>GGHMGAIVILVVGPPGSGKSQLIKAIEKLAREQGQPVVTTSVTSEDEAKKVLEELLKKDPNAIVVIEIKNPRIAERVAKRVLEEDPTAVLVVVVSSPEVARELRENLPNVIVVVLIRDPEKLKEAKKQGTQVLSGDGNPEEAAKQIAQLIKDQAGSWS[2x]

Here, we attempted to design an ATPase de novo, through the exploration of an optimal backbone blueprint to incorporate a conserved phosphate binding motif, the P‐loop, into designed structures. Many naturally occurring ATPases (Saraste et al., 1990; Walker et al., 1982) possess the P‐loop motif, with a sequence pattern of GX1X2X3X4GK[T/S] (X indicates any kind of amino acid residues). The P‐loop motifs in naturally occurring proteins typically show a cradle‐like conformation to grasp the phosphate moieties of the ATP molecule. The designed protein, based on the identified blueprint, was found to be a monomer with high thermal stability and exhibited ATPase ability.

The crystal structure of one of these designs, PL2x4_2, was determined and found to be nearly identical to the design model, both in overall structure and in the P‐loop motif. As a result, the blueprint with a 14‐residue helix, a loop with the AGBB ABEGO torsion pattern, and a six‐residue β‐strand was identified as the most optimal for allowing the Lys residue to point inward to the P‐loop cradle, facilitating the interaction with the β‐phosphate moiety. The P‐loop motif binds the phosphate group of the ATP molecule, while the adenine moiety is enclosed by a loop structure leading to the last helix. In this design, PL2x4_2, the adenine ring forms a hydrophobic interaction with Pro134 and two hydrogen bonds with Arg112 and Gln116. Arg112 is further stabilized by two hydrogen bonds with Gly11 in the P‐loop motif and Asp131. The de novo designed protein with the ideal P‐loop motif demonstrated ADP binding and ATP hydrolysis abilities as expected. However, these abilities are lower than those of typical naturally occurring ATPases. The simulations suggested that the low binding and hydrolysis activities might be due to a suboptimal binding pocket for the adenine and ribose moieties of ATP, as these moieties were detached from the binding pocket during the simulations. Furthermore, we found that the loop (the C‐terminal loop connected the sixth strand) adjacent to the binding pocket exhibited unsteady dynamic motion. Consistent with the simulations, each monomer in our crystal structure revealed different loop conformations, suggesting that the loop's flexibility might indeed contribute to the suboptimal binding pocket.>MGAAAKLAFAVFLISCSSGAILGRSETQECLFFNANWEKDRTNQTGVEPCYGDKDKRRHCFATWKNISGSIEIVKQGCWLDDINCYDRTDCVEKKDSPEVYFCCCEGNMCNEKFSYFPEME[4x];>[4x]GLECDGKVNICCKKQFFVSFKDIGWNDWIIAPSGYHANYCEGECPSHIAGTSGSSLSFHSTVINHYRMRGHSPFANLKSCCVPTKLRPMSMLYYDDGQNIIKKDIQNMIVEECGCS

Among type II receptors, TGFβR2 and AMHR2 only interact functionally with a select number of GFs, whereas ACVR2A, ACVR2B, and BMPR2 are promiscuous and can form signaling and nonsignaling complexes with an overlapping group of over 30 GFs, including homodimeric and heterodimeric activins, inhibins, bone morphogenetic proteins (BMPs), growth and differentiation factors (GDFs), Nodal, and Lefty. At the most basic level, TGF-β pathways are activated when a dimeric GF forms a signaling complex with both receptor types, triggering a phosphorylation cascade from receptors to R-SMADs that results in R-SMAD–mediated transcriptional responses. Structural and biochemical studies have revealed that the GF-binding domain (GBD) of both type I and type II receptors adopt a similar, “three-finger toxin fold”, where the “fingers” refer to three pairs of antiparallel β-strands that form an extended β-sheet. We have solved the crystal structures of the type II BMPR2 GBD in complex with activin B and of the type II activin Receptor ACVR2A in complex with activin A. We show that BMPR2 and activin type II receptors interact with GFs using a nearly identical mode of binding.

To identify molecular differences in GF recognition, we solved the structure of ACVR2A-GBD in complex with activin A and compared how the two receptors interact with these homologous GFs. For the ACVR2A complex, we used previous crystal structures as search models. The asymmetric unit of the BMPR2 complex comprised three receptor and three GF protomers, where all biological dimers were related by crystallographic symmetry. The asymmetric unit of the ACVR2A complex contained four receptor and four GF protomers, where all biological dimers were related by noncrystallographic symmetry (NCS). One significant difference between the two complexes is the relative orientation of GF protomers within a GF dimer. These differences can be attributed to flexibility of the activin dimer interface, which leads activin A to adopt a closed conformation and activin B an extended conformation. In addition, the different ACVR2A structures were completely superimposable, indicating that the conformational flexibility of the ACVR2A GBD is limited. Thus, BMPR2 has three extended loops linking strands β1–β2, β4–β5, and β5–β6 (blue circles), whereas ACVR2A has one extended loop linking strands β2–β3 (green circle). Notably, the GF-binding spectrum of ACVR2A was more stratified, with activin A, activin B, and GDF11 forming extremely stable complexes. However, the faster dissociation rate of activins A and B from BMPR2 indicated that activin–BMPR2 complexes are less stable than activin ACVR2A complexes, providing a rationale for the preferential utilization of ACVR2A by activins.> FNLDAEAPAVLSGPPGSFFGFSVEFYRPGTDGVSVLVGAPKANTSQPGVLQGGAVYLCPWGASPTQCTPIEFDSKGSRLLESSLSSSEGEEPVEYKSLQWFGATVRAHGSSILAC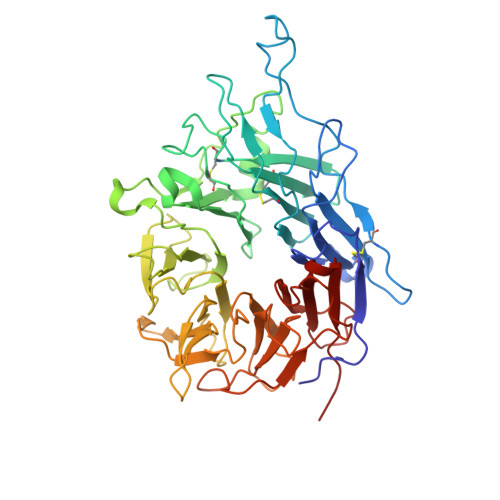APLYSWRTEKEPLSDPVGTCYLSTDNFTRILEYAPCRSDFSWAAGQGYCQGGFSAEFTKTGRVVLGGPGSYFWQGQILSATQEQIAESYYPEYLINLVQGQLQTRQASSIYDDSYLGYSVAVGEFSGDDTEDFVAGVPKGNLTYGYVTILNGSDIRSLYNFSGEQMASYFGYAVAATDVNGDGLDDLLVGAPLLMDRTPDGRPQEVGRVYVYLQHPAGIEPTPTLTLTGHDEFGRFGSSLTPLGDLDQDGYNDVAIGAPFGGETQQGVVFVFPGGPGGLGSKPSQVLQPLWAASHTPDFFGSALRGGRDLDGNGYPDLIVGSFGVDKAVVYRGRPVV>ANGLITKIWGTAGWTFNHAVTFGYPLNPTSDDKRRYKNYFISLGDVLPCRLCRESYKKFITTGKTALTN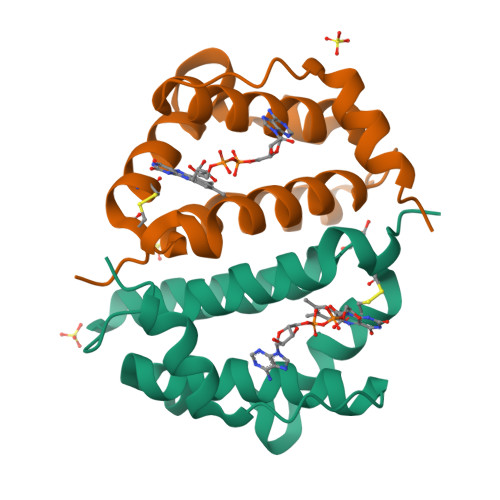EVLRNRHTLTKWFYDVHNAVNNKLEVDYGLSYEDVVNKYESFRAK[2x]>MSAQQPTIIYTLTDEAPLLATYAFLPVVRKFAEAAGIDVKTSDISVAARILAEFGDHLTEEQRVPDNLGELGALTQDPSANIIKLPNISASVPQLLAAIKELQGKGYNVPDYPANPKTDDEKKIKDRYAKILGSAVNPVLREGNSDRRAPKAVKEYARKHPHSMGEWSQASRTHVATMKTGDFYHGEKSMTLDRDRRVKMVLKTKSGEEIVLKPEVKLDAGDIIDSMYMSKKALIAFYEEQIEDAYKTGVMFSLHVKATMMKVSHPIVFGHAVKVFYKDAFAKHEKLFDELGVNVNNGLSDLYDKIEALPASQREEIIEDLHKCHEHRPELAMVDSAKGISNFHSPSDVIVDASMPAMIRLGGKMYGADGRTKDTKAVNPESTFSRMYQEMINFCKTHGQFDPTTMGTVPNVGLMAQKAEEYGSHDKTFEIPEDGVADIVDIDTGEVLLTQNVEEGDIWRMPIVKDAPIRDWVKLAVTRARLSGMPVVFWLDTERPHEVELRKKVKEYLKDHDTEGLKIQIMPQVWAMRYTLERVVRGKDTIAATGNILRDYLTDLFPILELGTSAKMLSIVPLMAGGGLY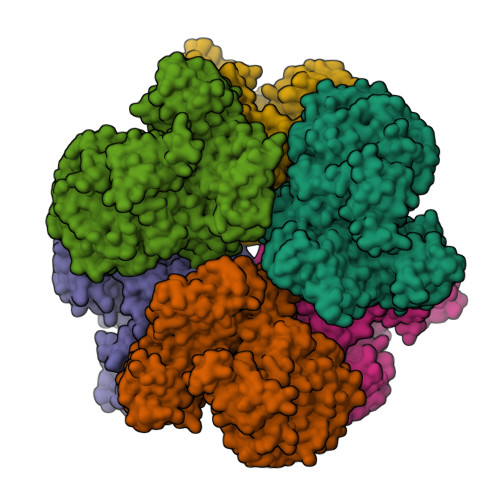ETGAGGSAPKHVHQLVEENHLRWDSLGEFLALGASLEDMGNKTGNEKAKVLAKALDTATGKLLEENKSPSRRTGELDNRGSQFYLSLFWAQALAEQTEDAELAERFKPLAKALAEQEEAIVSELNSVQGKTVDIGGYYYPDPEKTSEVMRPSKTFNTTLESVPRYPYDVPDYAKLAAALEHHHHHH[6x]> MTAEVMSHVTAHFGKTLEECREESGLSVDILDEFKHFWSDDFDVVHRELGCAIICMSNKFS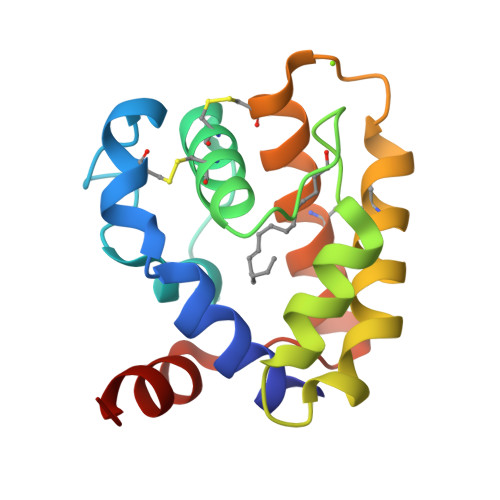LMDDDVRMHHVNMDEYIKSFPNGQVLAEKMVKLIHNCEKQFDTETDDCTRVVKVAACFKEDSRKEGIAPEVAMVEAVIEKY>TRDFNGTWEMESNENFEGYMKALDIDFATRKIAVRLTFTDVIDQDGDNFKTKATSTFLNYDVDFT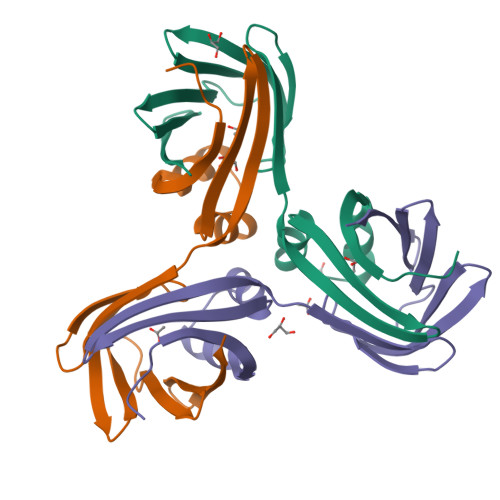VGVEFDEYTKSLDNRHVKALVTWEGDVLVCVQKGEKENRGWKKWIEGDKLYLELTCGDQVCRQVFKKK[6x]>MNLPTAQEVQGLMARY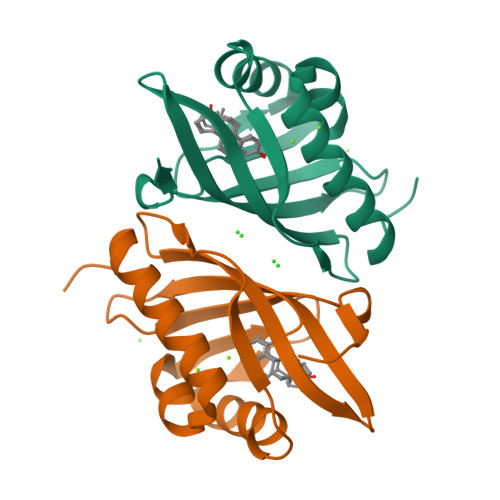IELVDVGDIEAIVQMYADDATVENPFGQPPIHGREQIAAFFRQGLGGGKVRACLTGPVRASHNGCGAMPFRVEMVWNGQPCALDVIDVMRFDEHGRIQTMQAYWSEVNLSVREPQ[2x]> MSAAPVLSITNASVVYPDGISTVTALDSANVEIFPGELVAIVGESGSGKSTLLSIAGFLQEPTSGTVTLHGAEGLDATSTRREHIGFVFQQPNLLGSLTAREQLLITDHLR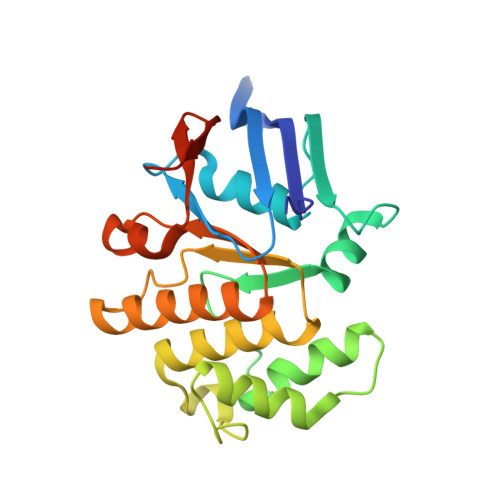GIKPRKDRADELLARVGLKGLGGRRVAQLSGGQRQRVNIARALMGNPQLLLADEPTSALDARLSKEIVELLRDVTKEFALATLMVTHDRSQLAYADRFVEMADGKALQTAKLWSHPQFEK(3S,4R)-3-hydroxy-2-oxopiperidin-4-yl beta-D-xylopyranoside 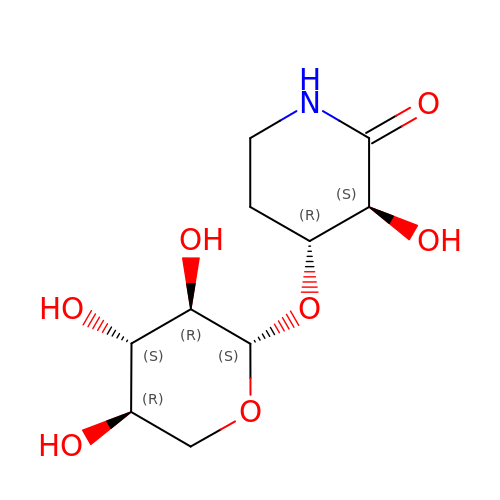| C10 H17 N O7 | BHZMHPRIYUPDCT-BQWZOORQSA-N> GHSKGRPQIDSSKATDK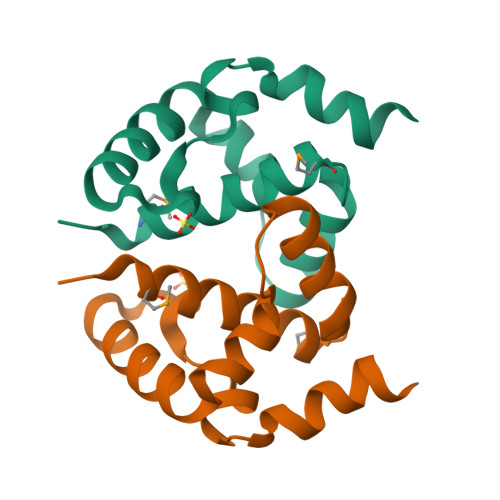INPMDFTFVEINEAVKLVEMGVATPQDIDTAIKLGLNRPFGPFELAKQFGAEQIAKRLEELAKQFGKKIFEPAKTLKEGKLEELLKAGKAEGS>[2x]SLKVNHTKSIGLLATSSEAAYFAEIIEAVEKNCFQKGYTLILGNAWNNLEKQRAYLSMMAQKRVDGLLVMCSEYPEPLLAMLEEYRHIPMVVMDFGEAKADFTDAVIDNAFEGGYMAGRYLIERGHREIGVIPGPLERNTGAGRLAGFMKAMEEAMIKVPESWIVQGDFEPESGYRAMQQILSQPHRPTAVFCGGDIMAMGALCAADEMGLRVPQDVSLIGYDNVRNARYFTPALT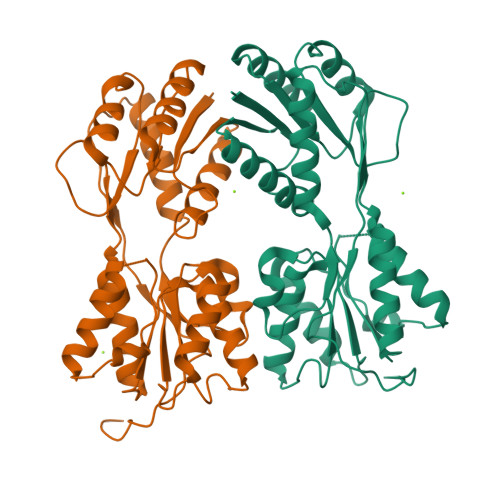TIHQPKDSLGETAFNMLLDRIVNKREEPQSIEVHPRLIERRSVADGPFRDYRR>ALTNAQILAVIDSWEETVGQFPVITHHVPLGGGLQGTLHCYEIPLAAPYGVGFAKNGPTRWQYKRTINQVVHRWGSHTVPFLLEPDNINGKTCTASHLCHNTRCHNPLHLCWESLDDNKGRNWCPGPNGGCVHAVVCLRQGPLYGPGATVAGPQQRGSHFVV[2x]

I-PpoI is a well-characterized intron-encoded homing endonuclease member of the physarum polycephalum slimemold. A large subfamily of one-metal-ion-dependent nucleases consist of histidine-metal (His-Me) nucleases that perform critical tasks in biological pathways such as apoptosis, extracellular defense, intracellular immunity (CRISPR–Cas9), and intron homing (homing endonuclease). Surrounded by two beta sheets and an alpha helix, the His-Me nucleases active sites all contain a single metal ion, a histidine, and an asparagine. The asparagine residue helps to stabilize metal ion binding whereas the strictly conserved histidine is suggested to deprotonate a nearby water for nucleophilic attack toward the scissile phosphate.

Next, we removed malonate in the crystallization buffer, which may chelate metal ions and hinder metal ion diffusion, by equilibrating the crystals in 200 mM NaCl buffer at pH 6, 7, or 8 for 30 min. The diffraction quality of the crystals was not affected during the soaking. The structures of I-PpoI equilibrated at pH 6, 7, or 8 in the presence of 200 mM NaCl showed no signs of product formation and appeared similar to the malonate and previous reported I-PpoI structures (Galburt et al., 1999; Flick et al., 1998). Within each I-PpoI active site, a water molecule (nucleophilic water, WatN) existed 3.6 Å from the scissile phosphate, near the imidazole side chain of His98. On the leaving group side of the scissile phosphate, the metal exhibited an octahedral geometry, being coordinated by three water molecules, two oxygen atoms from the scissile phosphate, and the conserved asparagine. Even in the absence of divalent Mg2+ or Mn2+, the active site including the scissile phosphate was already well aligned in I-PpoI, which is again different from RNaseH. During the reaction, the coordination distances of the metal ion ligands decreased 0.1–0.2 Å when Mg2+ exchanged with Na+, which is consistent with their preferred geometry (Cowan, 2002).> MVVIGEKFPEVEVKTTHGVIKLPDYFAEQGKWFVLFSHPADFTPVSTTEFYAMQKRVDQFRELGVEPIGLSVDQVCSHIKWMEWI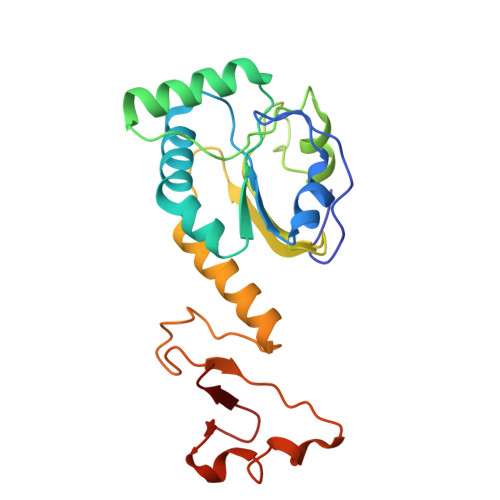KENLGEEITFPVIADDRGELADKLGMIPSGATITARAVFIVDDKGIIRAIVYYPAEVGRDWDEILRLVKALKVSDEKGVALPHKWPNNELIGDKAIVPPASTVDEVKQREEAKAKGEIESYDWWFSYKKLE The nuclear cap-binding complex (CBC) binds tightly to the 5′-cap structure (m7GpppN, where N is the first transcribed nucleotide) which is co-transcriptionally added to all nascent Pol II transcripts 25–50 nucleotides after initiation. CBC bound to capped RNA not only protects the transcript from decapping and subsequent further 5′-3′ degradation, but also acts as a platform for interaction with nuclear factors that determine the fate of the transcript. Here we take a biochemical and structural approach to investigate which binary and ternary complexes CBC can form with three nuclear factors, PHAX, ARS2 (arsenate resistance protein 2), and NELF (negative elongation factor), all of which directly interact with CBC and are involved in CBC-mediated transcript processing. We also determine crystal structures of CBC bound to ARS2 or NELF-E peptide that explain why CBC–ARS2–PHAX and CBC–NELF–E form mutually exclusive complexes.

The best results were obtained with CBC-NELF-E360–380 and m7GTP giving P21 monoclinic crystals that diffracted to 2.8 Å resolution. There are four m7GTP bound CBC complexes in the asymmetric unit with clear electron density for the NELF-E360–380 peptide in one of them (chain E) but weaker in the other copies. Remarkably the NELF-E and ARS2 C-terminal peptides bind to exactly the same site on m7GTP-CBC, at the interface of CBP20 and CBP80 and induce the same slight displacement of interacting regions of CBP20. The NELF-E peptide has a similar bipartite binding site to that of ARS2, with 360-DKRTQIVYSDDVYKE-372 in the proximal site and 378-DGF-380 in the distal site, and the bridging residues 375-NLV-377 poorly ordered. NELF-E Arg362 makes nearly identical interactions with CBP80 Tyr461 and CBP20 Gln55 and Asp107 as does Arg854 of ARS2 (left). NELF-E Tyr367 (which partially stacks on NELF-E Ile365) is buried in the same pocket as ARS2 Tyr859 (which partially stacks on ARS2 Val857), with its hydroxyl making an interaction with the side chain of CBP20 Glu53 (middle). Finally, there are highly analogous interactions of the NELF-E C-terminal Phe380 with CBP80 His651 as observed for ARS2 Phe871 (right). The major difference between NELF-E and ARS2 binding is that NELF-E has an additional tyrosine (Tyr372) which is buried in the interface. This tyrosine makes van der Waals contacts on one side with NELF-E Val371, and on the other side with CBP20 Ile70 and its hydroxyl group hydrogen bonds to the main-chain amino group of CBP20 Met71.

>MKTSDANETEDHLESLICKVGEKSACSLESNLEGLAGVLEADLPNYKSKILRLLCTVARLLPEKLTIYTTLVGLLNARNYNFGGEFVEAMIRQLKESLKANNYNEAVYLVRFLSDLVNCHVIAAPSMVAMFENFVSVTQEEDVPQVRRDWYVYAFLSSLPWVGKELYEKKDAEMDRIFANTESYLKRRQKTHVPMLQVWTADKPHPQEEYLDCLWAQIQKLKKDRWQERHILRPYLAFDSILCEALQHNLPPFTPPPHTEDSVYPMPRVIFRMFDYTDDPEGPVMPGSHSVERFVIEENLHCIIKSHWKERKTCAAQLVSYPGKNKIPLNYHIVEVIFAELFQLPAPPHIDVMYTTLLIELCKLQPGSLPQVLAQATEMLYMRLDTMNTTCVDRFINWFSHHLSNFQFRWSWEDWSDCLSQDPESPKPKFVREVLEKCMRLSYHQRILDIVPPTFSALCPANPTCIYKYGDESSNSLPGHSVALCLAVAFKSKATNDEIFSILKDVPNPNQDDDDDEGFSFNPLKIEVFVQTLLHLAAKSFSHSFSALAKFHEVFKTLAESDEGKLHVLRVMFEVWRNHPQMIAVLVDKMIRTQIVDCAAVANWIFSSELSRDFTRLFVWEILHSTIRKMNKHVLKIQKELEEAKEKLARQHKRRSDDDDRSSDRKDGVLEEQIERLQEKVESAQSEQKNLFLVIFQRFIMILTEHLVRCETDGTSVLTPWYKNCIERLQQIFLQHHQIIQQYMVTLENLLFTAELDPHILAVFQQFCALQA[4x];>[4x]GAMSGGLLKALRSDSYVELSQYRDQHFRGDNEEQEKLLKKSCTLYVGNLSFYTTEEQIYELFSKSGDIKKIIMGLDKMKKTACGFCFVEYYSRADAENAMRYINGTRLDDRIIRTDWDAGFKEGRQYGRGRSGGQVRDEYRQDYDAGRGGYGKLAQNQ;>DKRTQIVYSDDVYKENLVDGF[3x]>EPVMTGGPVQGKALWTDYSGMSKEVQGPVSQILFTQSPRTAKGDPYQNYPHYIPEGSRIVLFDLNTKELKVLTNDFATAFDPCTYWDGKKFAFAGVHKKGGGCQIWEMNIDGSGLRQMTDLKGTCRSPIYYAAGSIEEGEGRIIWRDRYFEGDWKEHGMVEKTGMIIFSGSPEGVMDEFHNPYAYNLYRLDTQGGKIIQRITGHVLSGIEFPHLNTTIDQITYNLSSNFDPWLTPDGNILFSSVQANGSRAGGEGRVMICVDNWDGAYPRPIYGNCDGEIGGTSGRSQAKITFGDRKIVYVESPYMNWGVGQLAAVSWDAPFNKTYEKLTGKDGGLYRSPYPLPDDRMLVSYAERGDFGIYWFNFSKCAAGDKVYDDPNWNDHQPAPVYVKYKPRWINTFTAGKNFGVTVVTYQPFDQVKVEGYPHSWGTWICFDTTLSDQPVGPYPHQKAKNVSHGDIKAVRIIQGYQCVEPDSTRFRVGAGAHLLGGERSSSNSGTAFQQRGIIGYQYVESDGSTVTSQLSDVPYYMQILDDKGMSVQTALTWAYLRPYHGRICSGCHYGSYRGRAFKNIHAKA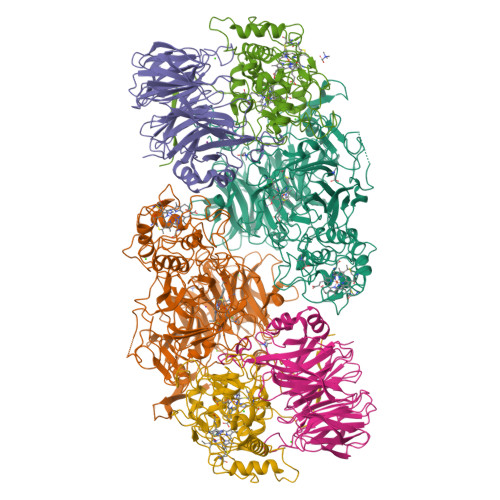LYNWWYDDRSHYDSPFAFRYLKFDNDGNYKGVKHGEDVVVPSDIYYGGPSGTTSQPVEGLTLDKQRTVDFRRDIQPILDAKCAMCHDSNNPPNLGGGLELVSVDGIAAYSRAYNSLLEPQRGKDPNIGGKYVNPSAAINSLLVWRLYEAELSANAPREKIFPIEGRLLHNKFLTQDERYAIVEWIDLGAQWDNIPGPDFYPGYLVK[2x];>GYIQGTHVKTDLPGPFHITMSPDGSTLFISNQSGHSVTFVDARTQKVTGEVAVRVQPEASAVTPDGAFLYVCNAESDSVSVVDIQRKQEIKEIKVGDWPSGIKISPDGKTAYVACSGCMWNAIDVIDTGRMEKVRSIYTSDYGPRMVEISPDGKTLVAILDTVGSINRSVDFIDIASGRVVENRVIHESSNLRDVVYTPDGKYIAVTHQTPKNWLPVCEAENGQVFTNNVTIIETKAGGKVARLPLDDLNNYDGNPYGMAMDPKGKYLYIGVRGMHRVTILDMDKVLGLVRSSTQEELDYLRDDLGLVRDYLVARVPTGLGPSSVCLSPDGKFCYAANYFSNNVTVIRTAVD[2x];>GQPRVISTIQTGATWEPLGREEPLTVPEVHFRVKHSPFKSELVRYGQFQFNDAAWSLQGSYSCASCHYERGQTTGLIWDLGDEGWGSWKNTKYIRGGRYLPPFRHEGFTGHPDEIVGATSSLDRVCGRDPGFVFRSENFSPMRLEALICYIRALEFTGSPFRNADGSLTEAQKRGQKIFEDPKVGCLECHPGDPMDPRALFSDAQTHDVGTGRVGVNGFRSTPGKVFNISALEAGEDPYGVESNTPIIGLDLVKEFDTPTLRDIYASGTYFHDGGARTLMDTINNTVNDKDMHGRTSHLKQQELQDLVEYLKAL[2x]> GPHMRTFFVGGNWKANPKTVQEAEKLVEML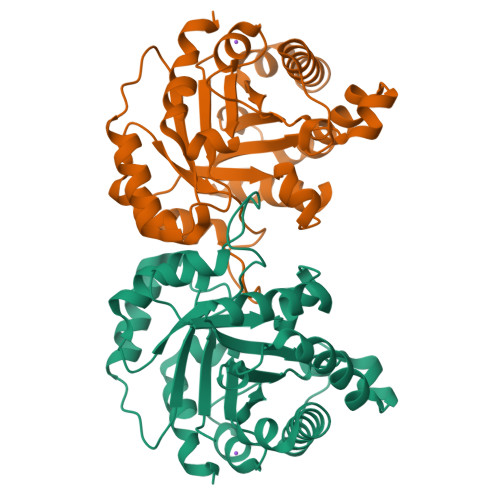NGAKVEGNVEVVVAAPFVFLPTLQQKLRKDWKVSAENVFTKPNGAFTGEVTVPMIKSFGIEWTILGHSERRDILKEDDEFLAAKAKFALENGMKIIYCCGEHLSEREAGKASEFVSAQIEKMIPAIPAGKWDDVVIAYEPIWAIGTGKVASTQDAQEMCKVIRDILAAKVGADIANKVRILYGGSVKPNNCNELAACPDVDGFLVGGASLEAGFINIVNSNVHSK> PLPPLPPLPPLPPLPP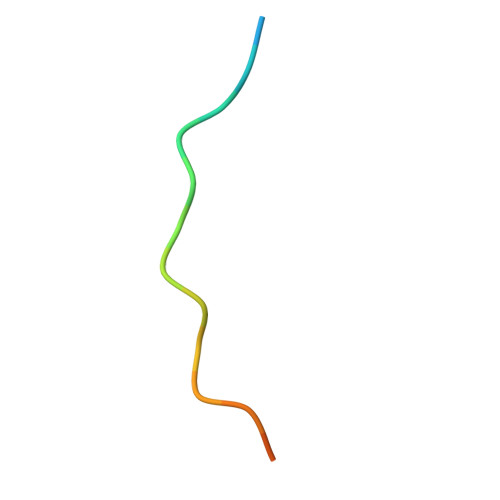LP> MSEEILFDCLHAEIVNYCLDSNKEHDLATLEYIGFTTGYRLIERLTREVSRFKDELETMKFICTDFWMLIYKKQVDNLRTNNHGMYVVQDKAFRFLTRISPGTKQLEHAPKFVAFTCGLVRGALSNLGINSTVTAEVQSIPACKFHI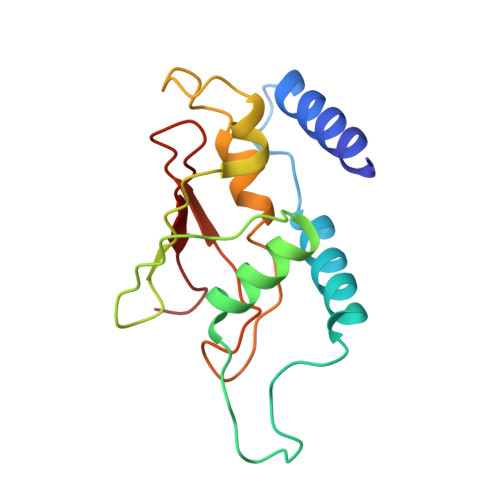EVNRN>MGRDPNSTNDTTTQNVVLTKYGFDKDVTAIDRATDQIWTGDGAKPLQGVDFTIYNVTANYWASPKDYKGSFDSAPVAATGTTNDKGQLTQALPIQSKDASGKTRAAVYLFHATNPRAGYNTSADFWLTLPAKAAADGNVYVYPKNVQKTTYERTFVKKDAETKEVLEGAGFKISNSDGKFLKLTDKDGQSVSIGEGFIDVLANNYRLTWVAESDATV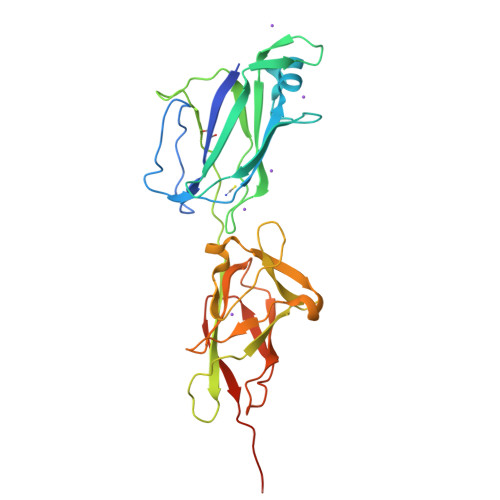FTSDKSGKFGLNGFADNTTTYTAVETNVPDGYDAAANTDFKADNSSSDILDAPSGILPLEHHHHHH[3x]> TRPNHTIYINNLNSKIKKDELKKSLHAIFSRFGQILDILVPRTRRPRGQAFVIFKEVSSATNALRSMQGFPFYDKPMAIQYAKTDRTI

The viral trans-activator of transcription (Tat) protein uses an archetypal arginine-rich motif (ARM) to recruit the host positive transcription elongation factor b (pTEFb) complex onto the viral trans-activation response (TAR) RNA, leading to activation of HIV transcription. Using yeast display and multiple rounds of selection, a new class of TAR-binding proteins (TBPs) was identified that bind TAR with nanomolar affinity. Here, we present four co-crystal structures of lab-evolved TAR-binding proteins (TBPs) in complex with HIV-1 TAR. Although it was hypothesized originally that each TBP variant would recognize TAR using fundamentally different modes of binding, we demonstrated here that each TBP binds TAR using a conserved subset of arginine-to-guanine interactions within a lab-evolved β2-β3 loop.

To examine the role of arginine placement in TAR recognition, we first considered TBP6.3, which differs from TBP6.7 by the change of Q48T and T50R. ITC analysis showed a KD of 45.2 ± 3.4 nm for TBP6.3, representing a ΔΔG° of +1.2 kcal mol−1 compared with TBP6.7—signifying a less favorable binding equivalent to ∼2 hydrogen bonds (Krel of 8-fold). However, we observed that Arg-50 of TBP6.3 displaced Arg-52, usurping its role in Gua36 recognition. Arg-52 adopted a new conformation that protrudes into the TAR bulge to interact with the backbone at the pro-Rp oxygen of Uri23. Thr-48 had no deleterious effects except that its side chain is too short to hydrogen-bond with the phosphate backbone as observed for Gln-48 in TBP6.7. Although TBP6.3 contains four arginines, this variant exhibited 8.5-fold weaker binding than TBP6.7, which has three β2-β3 loop arginines. Although TBP6.3 contains four arginines like TBP6.9, the former exhibits two suboptimal interactions. Namely, the Arg-50 guanidinium is not co-planar with the Gua36 base, yielding a weak inclined hydrogen bond interaction to the base Hoogsteen edge. Similarly, accommodation of Arg-50 in place of Arg-52 pulls nearby Arg-49 away from the phosphate backbone such that the Arg-49 guanidium group hydrogen-bonds to O6 and N7 of Gua28 rather than N7 and the Gua28 phosphate—as observed in TBP6.9. In contrast, TBP6.3 cannot form this interaction because Thr-50 was replaced by Arg-50.> MKALVRLSSNHIFRSDSMSRVWLTGDAVVDLIPDGQQHYLKCPGGAPANVAVAIARLSGRSAFFGRVGNDPFGRFMQQTLTDEQVDCQHLHFDPVHRTSTVVV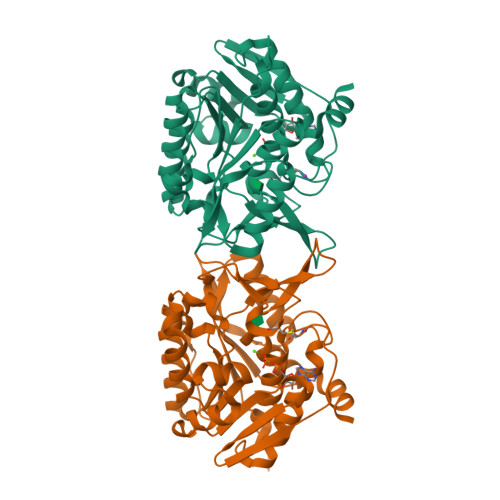DLDECGERSFTFMVKPSADQFLQLSDIPSFQKGEWLHVCSIALANQPSRSSTFAAIAQMKEVGGYVSFDPNLREEVWSEPQELQATVMRAVGLADVVKFSEEELQFLTGTQSIEEGLQAIADFQIPLVVVTLGAKGALVATPNSQQIVSGKAVKPIDCTGAGDAFVGGLLYRLSVAQDWHNQATILDAVKWANGCGALATTQKGAMTALPNQAALYAFLE> SDRAEVRNIPFKLGMYLTVGGVVNSNATRF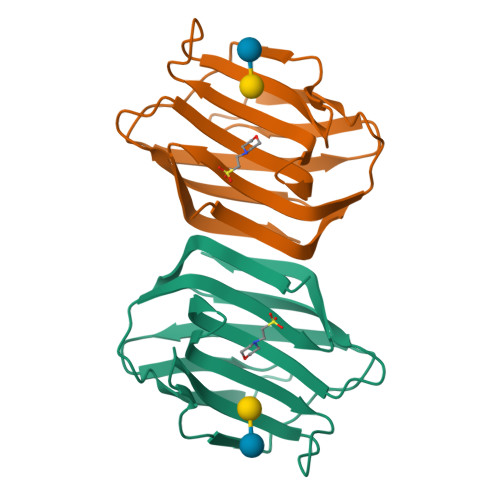SINVGESTDSIAMHMDHRFSYGADQNVLVLNSLVHNVGWQQEERSKKFPFTKGDHFQTTITFDTHTFYIQLSNGETVEFPNRNKDAAFNLIYLAGDARLTFVRLE>SNASRSYNDELQFLEKINKNCWRIKKGFVPNMQVEGVFYVNDALEKLMFEELRNACRGGGVGGFLPAMKQIGNVAALPGIVHRSIGLPDVHSGYGFAIGNMAAFDMNDPEAVVSPGGVGFDINCGVRLLRTNLDESDVQPVKEQLAQAMFDHIPVGVGSKGVIPMNAKDLEEALEMGVDWSLREGYAWAEDKEHCEEYGRMLQADPNKVSARAKKRGLPQLGTLGAGNHYAEIQVVDEIFNEYAAKKMGIDHKGQVCVMIHSGSRGLGHQVATDALVAMEKAMKRDKIIVNDRQLACARIASPEGQDYLKGMAAAGNYAWVNRSSMTFLTRQAFAKVFNTTPDDLDLHVIYDVSHNIAKVEQHVVDGKERTLLVHRKGSTRAFPPHHPLIAVDYQLTGQPVLIGGTMGTCSYVLTGTEQGMTETFGTTCHGAGRALSRAKSRRNLDFQDVLDKLADMGIAIRVASPKLVMEEAPESYKNVTDVVNTCHDAGISKKAIKLRPIAVIKG[2x]

The human RtcB ligase ortholog RTCB, also referred to as HSPC117 or FAAP, is part of an essential heteropentameric tRNA ligase complex (tRNA-LC), along with the DEAD-box helicase DDX1, as well as FAM98B, CGI-99 (also known as RTRAF or hCLE), and ASHWIN (ASW). The tRNA ligase complex is an essential factor for both tRNA biogenesis and XBP1 mRNA splicing during the unfolded protein response in human cells. By contrast, the RtcB ligases are GTP-dependent enzymes that catalyze the direct joining of RNA strands with terminal 2′,3′>P and 5′-OH. RTCB is the only subunit of tRNA-LC that is essential and sufficient for RNA ligation, but it requires the protein cofactor Archease for multiple-turnover catalysis.

To address this, we determined, at a resolution of 2.3 Å, the crystal structure of human RTCB in complex with a GMP molecule and two divalent cobalt ions bound in the active site. The structure of GMP-bound RTCB likely mimics an on-pathway, product-bound state. The GMP guanosine base makes hydrogen bonding interactions with the sidechains of Glu230RTCB, Ser409RTCB, and Lys504RTCB. The ribose 2′ and 3′ OH groups are hydrogen-bonded with backbone nitrogens of Ala430RTCB and Gly431RTCB, while the phosphate oxygen atoms interact with the sidechains of Asn226RTCB and His428RTCB. The phosphate moiety is further coordinated by the Co2+(A) ion. The two Co2+ ions, referred to as Co2+(A) and Co2+(B), adopt tetrahedral and octahedral coordination geometries, respectively. Co2+(A) is coordinated by His259RTCB, His353RTCB, Cys122RTCB, and the phosphate moiety of GMP, whereas Co2+(B) is coordinated by Asp119RTCB, Cys122RTCB, His227RTCB, and three water molecules. Two adjacent loops found in the vicinity of the active site in RTCB are structurally distinct from PhRtcB: an N-terminal region spanning residues Leu45-Pro64RTCB, which forms an extended α-helix and a loop as compared to a shorter loop (Lys37-Arg42PhRtcB) in PhRtcB, and a segment comprising residues Arg436-Asp444RTCB, which is only partially ordered. The RTCB structure shows that the metal ion A is tetrahedrally coordinated, instead of adopting octahedral coordination as observed in the Mn2+-bound PhRtcB structures. Unlike the prokaryotic RtcB orthologs, human RTCB is active in the presence of Co2+ ions, suggesting that the Co2+-bound RTCB structure represents an on-pathway state and not a catalytically inhibited complex.> QDADKLPHTKVTLVAPPQVHPHEQASKTGPKVVEFTMTIEEKKMVIDDKGTTLQAMTFNGSMPGPTLVVHEGDYVQLTLVNPATNAMPHNVDFHGATGALGGAKLTNVNPGEQATLRFKADRSGTFVYHCAPEGMVPWHVVSGLSGTLMVLPRDGLKDPEGKPLHYDRAYTIGEFDLYIPKGPDGKYKDYATLAESYGDTVQVMRTLTPSHIVFNGKVGALTGANALTAKVGETVLLIHSQANRDTRPHLIGGHGDWVWETGKFANPPQRDLETWFIRGGSAGAALYTFKQPGVYAYLNHNLIEAFELGAAGHIKVEGKWNDDLMKQIKAPAPIPR;> QDADKLPHTKVTLVAPPQVHPHEQATKSGPKVVEFTMTIEEKKMVIDDKGTTLQAMTFNGSMPGPTLVVHEGDYVQLTLVNPATNAMPHNVDFHGATGALGGAKLTNVNPGEQATLRFKADRSGTFVYHCAPEGMVPWHVVSGLSGTLMVLPRDGLKD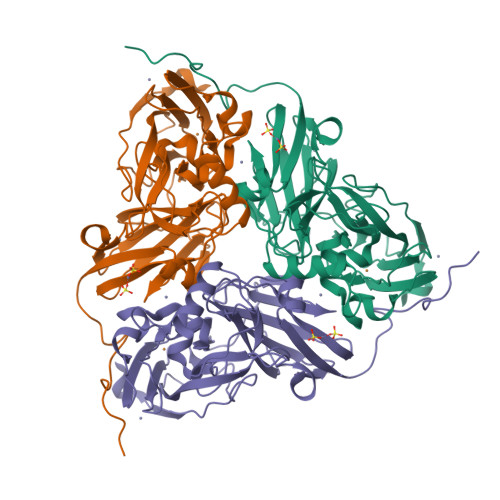PEGKPLHYDRAYTIGEFDLYIPKGPDGKYKDYATLAESYGDTVQVMRTLTPSHIVFNGKVGALTGANALTAKVGETVLLIHSQANRDTRPHLIGGHGDWVWETGKFANPPQRDLETWFIRGGSAGAALYTFKQPGVYAYLNHNLIEAFELGAAGHIKVEGKWNDDLMKQIKAPAPIPR> MEKTTEGAFYTREYRNLFKEFGYSEAEIQERVKDTWEQLFGDNPETKIYYEVGDDLGYLLDTGNLDVRTEGMSYGMMMAVQMDRKDIFDRIWNWTMKNMYMTEGVHAGYFAWSCQPDGTKNSWGPAPDGEEYFALALFFASHRWGDGDEQPFNYSEQARKLLHTCVHNGEGGPGHPMWNRDNKLIKFIPEVEFSDPSYHLPHFYELFSLWANEEDRVFWKEAAEASREYLKIACHPETGLAPEYAYYDGTPNDEKGYGHFFSDSYRVAANIGLDAEWFGGSEWSAEEINKIQAFFADKEPEDYRRYKIDGEPFEEKSL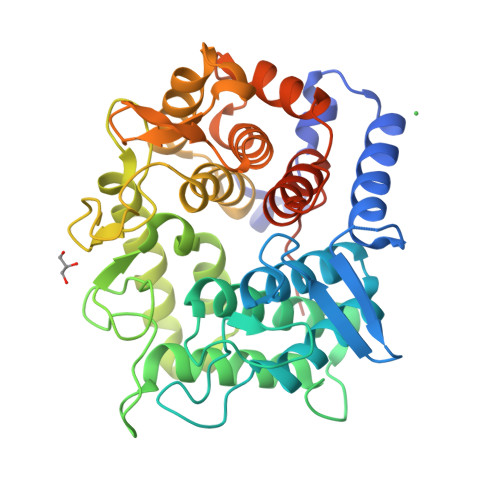HPVGLIATNAMGSLASVDGPYAKANVDLFWNTPVRTGNRRYYDNCLYLFAMLALSGNFKIWFPEGQEEEHLEHHHHHH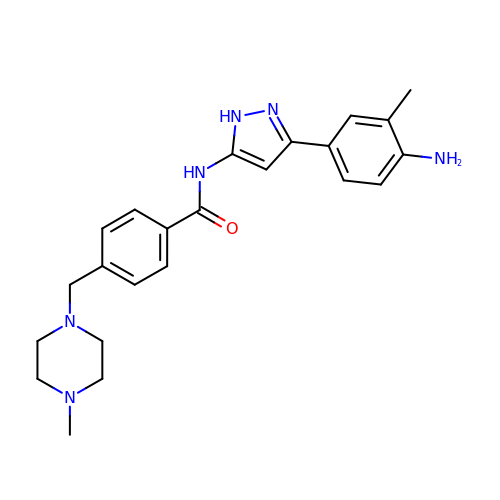N-[3-(4-amino-3-methylphenyl)-1H-pyrazol-5-yl]-4-[(4-methylpiperazin-1-yl)methyl]benzamide | C23 H28 N6 O | BUBLMWQDUODHGD-UHFFFAOYSA-N>[4x]GAMTAEALELGRQQAQLLRRSVRRFSTDPVPGDLVEAAVAEALTAPAPHHTRPTRFVWLQTPAIRARLLDRMKDKWRSDLTS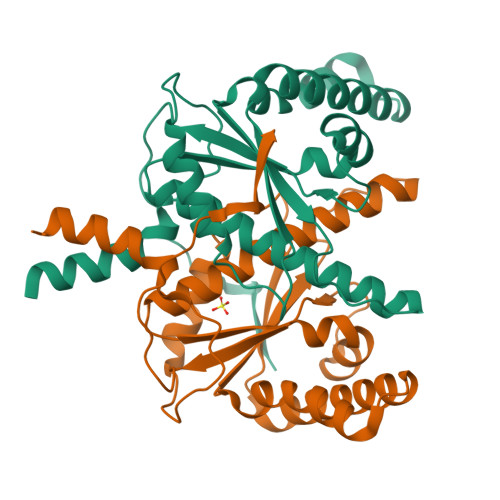DGLPADAIERRVARGQILYDAPEVVIPMLVPDGAHSYPDAARTDAEHTMFTVAVGAAVQALLVALAVRGLGSCWIGSTIFAADLVRDELDLPVDWEPLGAIAIGYADEPSGLRDPVPAADLLILK>EFNPLCFECGQQHWTRENHLYNYQNEVDD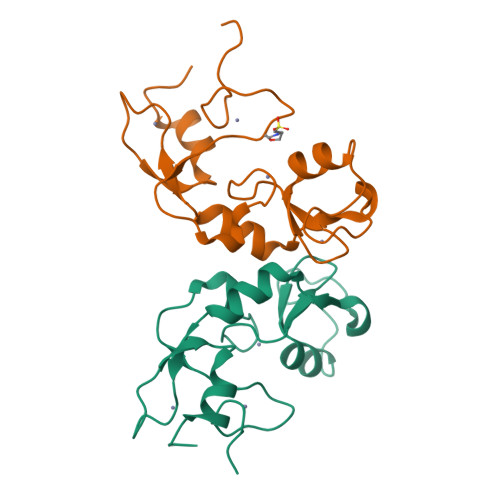DLVCHICLQPLLQPLDTPCGHTFCYKCLRNFLQEKDFCPLDRKRLHFKLCKKSSILVHKLLDKLLVLCPFSSVCKDVMQRCDLEAHLKNRCPGASHRRVAL[2x]> MKGSRIELGDVTPHNIKQLKRLNQVIFPVSYND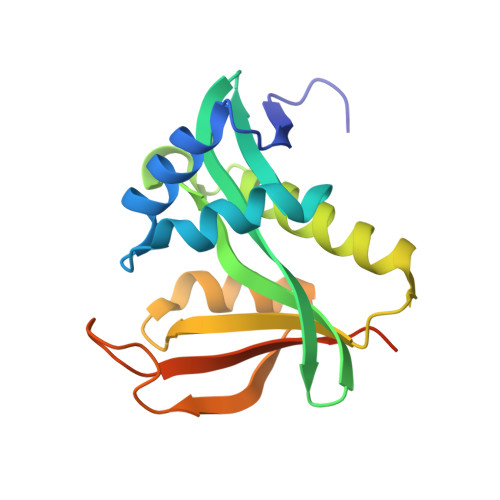KFYKDVLEVGELAKLAYFNDIAVGAVCCRVDHSQNQKRLYIMTLGCLAPYRRLGIGTKMLNHVLNICEKDGTFDNIYLHVQISNESAIDFYRKFGFEIIETKKNYYKRIEPADAHVLQKNLKVPSGQNADVQKTDN>GHMATGTRYAGKVVVVTGGGRGIGAGIVRAFVNSGARVVICDKDESGGRALEQELPGAVFILCDVTQEDDVKTLVSETIRRFGRLDCVVNNAGHHPPPQRPEETSAQGFRQLLELNLLGTYTLTKLALPYLRKSQGNVINISSLVGAIGQAQAVPYVATKGAVTAMTKALALDESPYGVRVNCISPGNIWTPLWEELAA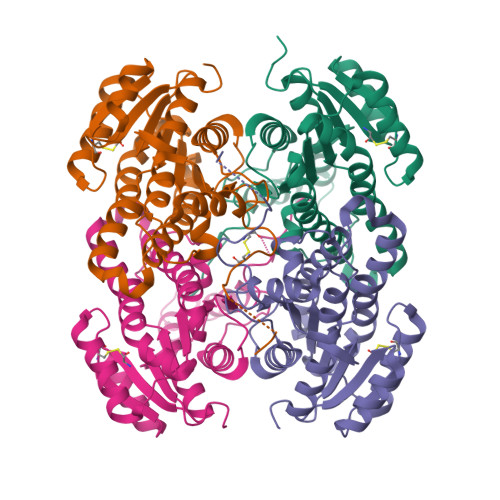LMPDPRASIREGMLAQPLGRMGQPAEVGAAAVFLASEANFCTGIELLVTGGAELGYGCKASRSTPVDAPDIPSGS[4x]Thioredoxins (TRXs) are small oxidoreductases that contribute, in most living organisms, to the control of cellular redox homeostasis. Indeed, they reduce disulfide bonds on numerous proteins involved in several processes, including antioxidant defense mechanisms, photosynthetic carbon metabolism, and protein folding. In addition, TRXs have been suggested to control two additional Cys-based post-translational modifications, namely S-glutathionylation and S-nitrosylation, by catalyzing the reduction of glutathione-mixed disulfides (–SSGs) and S-nitrosothiols (–SNOs), respectively. The redox activity of TRXs relies on the presence of two Cys residues in the conserved Trp-Cys-(Gly/Pro)-Pro-Cys (WC(G/P)PC) active site motif.

In the present study, we deepen the structural features of CrTRXh1, providing the 3D structures of both the reduced form and variants in which catalytic cysteines were mutated. Structural alignments and circular dichroism (CD) analysis of reduced and oxidized CrTRXh1 reveal an identical folding independent on the redox state. The analysis of the catalytic site microenvironment from the crystal structure of reduced CrTRXh1 indicates that a hydrogen-bonding network is the major factor determining CysN reactivity. Through mass spectrometry (MS) analysis coupled to pH-dependent iodoacetamide (IAM)-based alkylation, we experimentally determined the pKa of both active site cysteines.

>MGGSVIVIDSKAAWDAQLAKGKEEHKPIVVDFTATWCGPCKMIAPLFETLSNDYAGKVIFLKVDVDAVAAVAEAAGITAMPTFHVYKDGVKADDLVGASQDKLKALVAKHAAA[2x]> QSESYKDAYSRINAIVIEGEQEAFDNYNRLAEMLPDQRDELHKLAKMEQRHMKGFMACGKNLSVTPDMGFAQKFFERLHENFKAAAAEGKVVTCLLIQSLIIECFAIAAFNIYIPVADAFARKITEGVVRD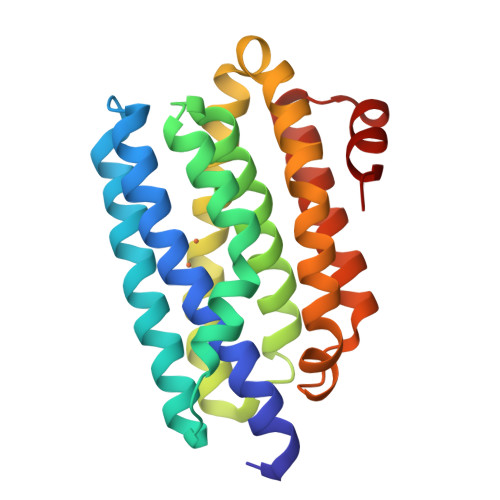EYLHRNFGEEWLKANFDASKAELEEANRQNLPLVWLMLNEVADDARELGMERESLVEDFMIAYGEALENIGFTTREIMRMSAYG;> SYKDAYSRINAIVIEGEQEAFDNYNRLAEMLPDQRDELHKLAKMEQRHMKGFMACGKNLSVTPDMGFAQKFFERLHENFKAAAAEGKVVTCLLIQSLIIECFAIAAFNIYIPVADAFARKITEGVVRDEYLHRNFGEEWLKANFDASKAELEEANRQNLPLVWLMLNEVADDARELGMERESLVEDFMIAYGEALENIGFTTREIMRMSAYG> GSGKSLLLKVILLGDGGVGKSSLMNRYVTNKFDSQAFHTIGVEFLNRDLEVDGRFVTLQIWDTAGQERFKSLRTPFYRGADCCLLTFSVDDRQSFENLGNWQKEFIYYADVKDPEHFPFVVLGNKVDKEDRQVTTEEAQTWCMENGDYPYLETSAKDDTNVTVAFEE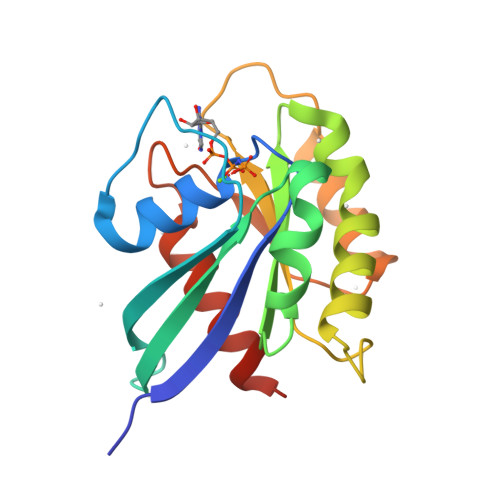AVRQVLAVEEQLE> DKAMAGNFWQSSHYLQWILDKQDLLKERQKDLKFLSEEEYWKLQIFFTNVIQALGEHLKLRQQVIATATVYFKRFYARYSLKSIDPVLMAPTCVFLASK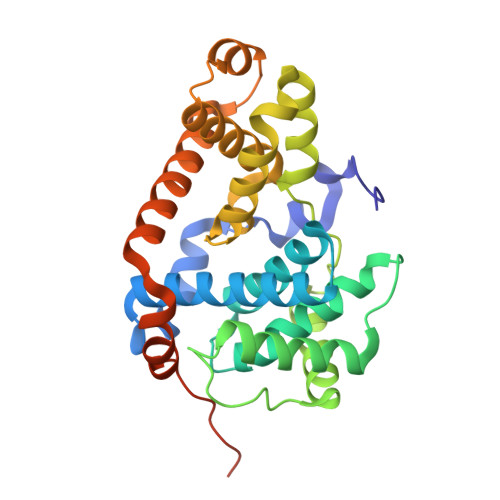VEEFGVVSNTRLIAAATSVLKTRFSYAFPKEFPYRMNHILECEFYLLELMDCCLIVYHPYRPLLQYVQDMGQEDMLLPLAWRIVNDTYRTDLCLLYPPFMIALACLHVACVVQQKDARQWFAELSVDMEKILEIIRVILKLYEQWKNFDERKEMATILSKMPKPKPPPNSEGEQGPNGSQNSSY> TVGAVALDLDGNLAAATSTGGMTNK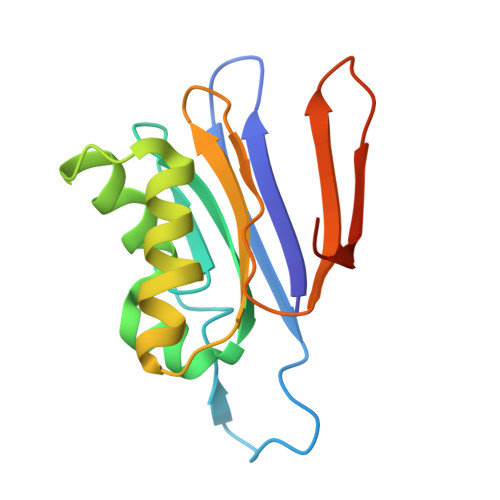LPGRVGDSPLVGAGCYANNASVAVSCTGTGEVFIRALAAYDIAALMDYGGLSLAEACERVVMEKLPALGGSGGLIAIDHEGNVALPFNTEGMYRAWGYAGDTPTTGIYREKGDTVATQ>[12x]MSEFVSIAARQEGAVGIIELARPDVLNALSRQMVAEIVAAVEAFDRNEKVRVIVLTGRGRAFAAGADIQEMAKDDPIRLEWLNQFADWDRLSIVKTPMIAAVNGLALGGGFELALSCDLI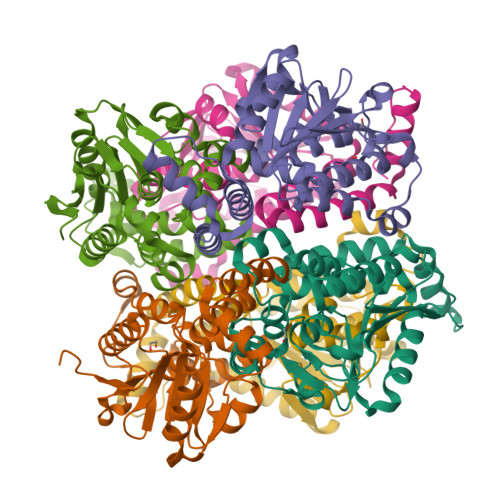VASSAAEFGFPEVNLGVMPGAGGTQRLTKLIGPKRALEWLWTGARMSAKEAEQLGIVNRVVSPELLMEETMRLAGRLAEQPPLALRLIKEAVQKAVDYPLYEGMQFERKNFYLLFASEDQKEGMAAFLEKRKPRFQGK> G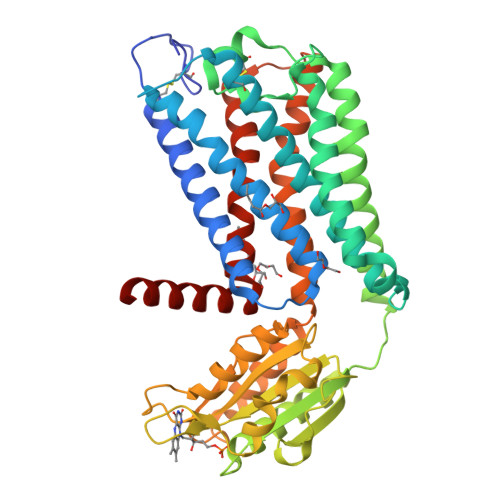GIVNVSERHSCPLGFGHYSVVDVCIFETVVIVLLTFLIIAGNLTVIFVFHCAPLLHHYTTSYFIQTMAYADLFVGVSCLVPTLSLLHYSTGVHESLTCQVFGYIISVLKSVSMWCLACISVDRYLAITKPLSYNQLVTPCRLRICIILIWIYSCLIFLPSFFGWGKPGYHGDIFEWCATSWLTSAYFTGFIVCLLYAPAAFVVCFTYFHIFKICRQHTKEAKALIVYGSTTGNTEYTAETIARELADAGYEVDSRDAASVEAGGLFEGFDLVLLGCSTWGDDSIELQDDFIPLFDSLEETGAQGRKVACFGCGDSSWEYFCGAVDAIEEKLKNLGAEIVQDGLRIDGDPRAARDDIVGWAHDVRGAIRRYLMVLFRITSVFYMLQLPYIIYFLLESSRVLDNPTLSFLTTWLAISNSFCNPVIYALSDSTFRLGLRRLSETMCTSCMC BusR is a member of a yet structurally uncharacterized subfamily of the GntR family of transcription factors that downregulates transcription of the genes for the BusA (OpuA) glycine-betaine transporter upon c-di-AMP binding. BusR satisfies the overall domain architecture of the GntR family with its N-terminal winged helix-turn-helix motif (wHTH) and a C-terminal effector binding motif, an RCK_C domain (regulator of K+ conductance). Our structural data, supported by biochemical and biophysical data, reveal that BusR utilizes a unique domain assembly with a tetrameric coiled-coil in between the binding platforms, serving as a molecular ruler to specifically recognize a 22 bp separated bipartite binding motif. Binding of c-di-AMP to BusR induces a shift in equilibrium from an inactivated towards an activated state that allows BusR to bind the target DNA, leading to transcriptional repression.

We purified and crystallized a construct comprising only the RCK_C domain (Leu135 to end) and solved its ligand-free and c-di-AMP bound structure to 1 and 1.2 Å resolution, respectively. The crystal of the apo state only contains one monomer in the asymmetric unit. However, a symmetry related copy is present that generates the dimeric assembly as common to RCK_C domains and as observed in our full-length structure. The scattering data show that the RCK_C domain on its own is dimeric in solution even in the absence of c-di-AMP. The apo and c-di-AMP bound crystal structure of the RCK_C domain show that c-di-AMP binding induces a subtle rotation of the RCK_C domains that results in a widening of the binding pocket. This movement pushes residues Pro179, Gly180, Pro181 and Phe182 (chain A) further out in respect to Trp159 (chain B) of the opposing chain. Thus, it seems that this interface locks wHTHinhib in an autoinhibited state in absence of c-di-AMP, restricting movement of wHTHinhib and thus impairing high affinity binding to the operator sequence.

> MAHHHHHHSAALEVLFQGPLAPYEIIVSEDSEHLGKSIGELNVWHQTGATIVAIEHEGKFIVSPGPFSVIEQGDHIFFVGDEDVYARMKTYFNLRMGL> MINIDRRRKDIIRTININPTNITITSIKKTE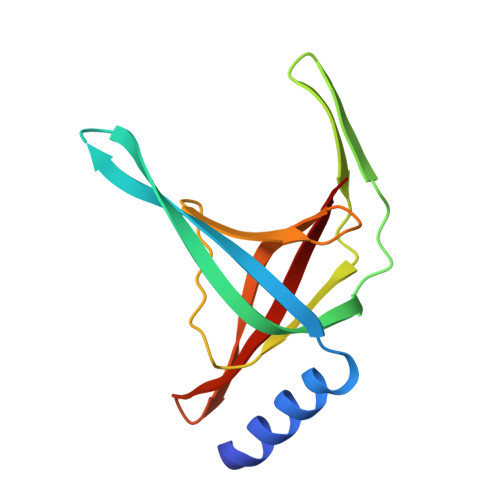IDGAFEETETEIKCVVRIFNEKTAEKQISSEKQGTFSSIRTYGMLVSNDVILEVNSRDSLEFECIYGRMKIVNIYPQIVKGELCGYQCSLERID>[2x]MAETQFTRFPFQPFII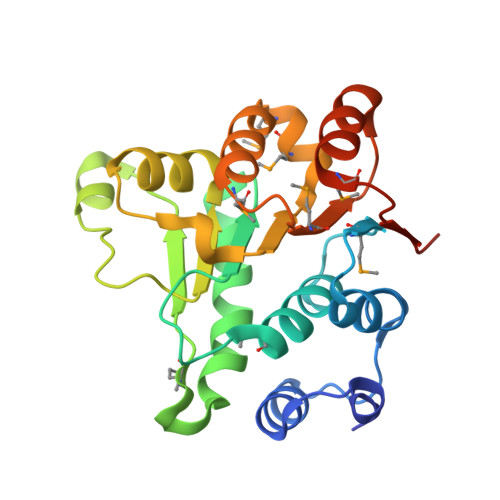EAIKTLRFYKPTEIQERIIPGALRGESMVGQSQTGTGKTHAYLLPIMEKIKPERAEVQAVITAPTRELATQIYHETLKITKFCPKDRMIVARCLIGGTDKQKALEKLNVQPHIVIGTPGRINDFIREQALDVHTAHILVVDEADLMLDMGFITDVDQIAARMPKDLQMLVFSATIPEKLKPFLKKYMENPTFVHVLEHHHHHH thiolane 1-oxide | C4 H8 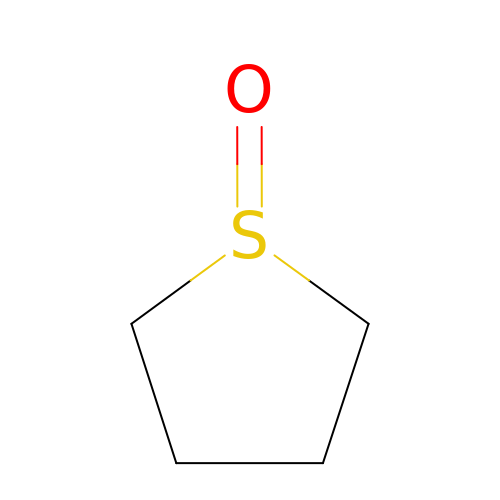O S | ISXOBTBCNRIIQO-UHFFFAOYSA-N>MENFKHLPEPFRIRVIEPVKRTTRAYREEAIIKSGMNPFLLDSEDVFIDLLTDSGTGAVTQSMQAAMMRGDEAYSGSRSYYALAESVKNIFGYQYTIPTHQGRGAEQIYIPVLIKKREQEKGLDRSKMVAFSNYFFDTTQGHSQINGCTVRNVYIKEAFDTGVRYDFKGNFDLEGLERGIEEVGPNNVPYIVATITSNSAGGQPVSLANLKAMYSIAKKYDIPVVMDSARFAENAYFIKQREAEYKDWTIEQITRETYKYADMLAMSAKKDAMVPMGGLLCMKDDSFFDVYT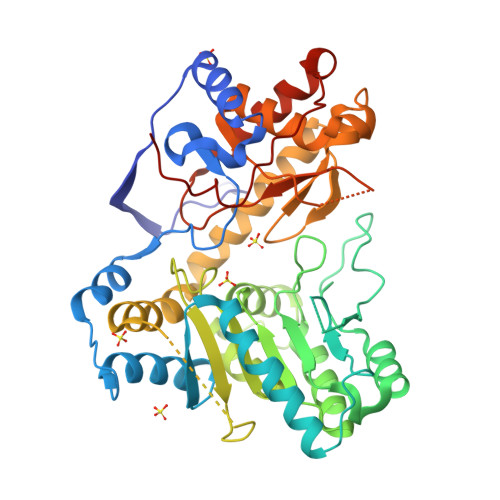ECRTLCVVQEGFPTYGGLEGGAMERLAVGLYDGMNLDWLAYRIAQVQYLVDGLEEIGVVCQQAGGHAAFVDAGKLLPHIPADQFPAQALACELYKVAGIRAVEIGSFLLGRDPKTGKQLPCPAELLRLTIPRATYTQTHMDFIIEAFKHVKENASNIKGLTFTYEPKVLRHFTAKLKEV[4x]>GSHMASFNGVSEAELLTKTLPDILTFNLDIVIIGINPGLMAAYKGHHYPGPGNHFWKCLFMSGLSEVQLNHMDDHTLPGKYGIGFTNMVERTTPGSKDLSSKEFREGGRILVQKLQKYQPRIAVFNGKCIYEIFSKEVFGVKVKNLEFGLQPHKIPDTETLCYVMPSSSARCAQFPRAQDKVHYYIKLKDLRDQLKG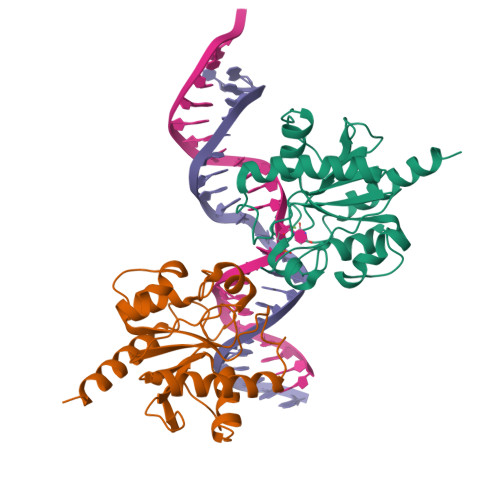IERNMDV[2x]>[2x]QLTIEVLVTVDGVNFRTVVLNNKNTYRSQLGCVFFNGADISDTIPDEKQNGHSLYLADNLTADETKALKELYGPVDPTFLHRFYSLKAAVHGWKMVVCDKVRSLKLSDNNCYLNAVIMTLDLLKDIKFVIPALQHAFMKHKGGDSTDFIALIMAYGNCTFGAPDDASRLLHTVLAKAELCCSARMVWREWCNVCGIKDVVLQGLKACCYVGVQTVEDLRA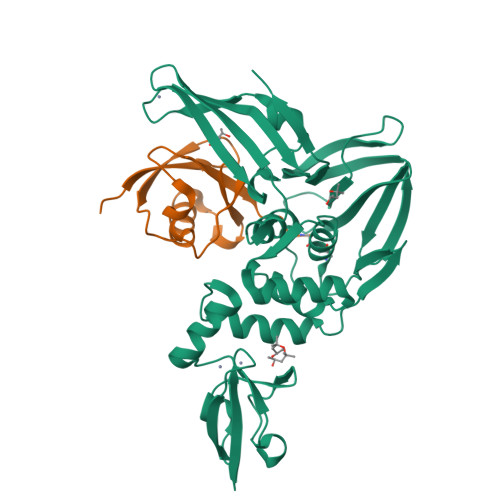RMTYVCQCGGERHRQLVEHTTPWLLLSGTPNEKLVTTSTAPDFVAFNVFQGIETAVGHYVHARLKGGLILKFDSGTVSKTSDWKCKVTDVLFPGQKYSSDCN;>MEPLSILVRNNKGRSSTYEVRLTQTVAHLKQQVSGLEGVQDDLFWLTFEGKPLEDQLPLGEYGLKPLSTVFMNLRLRG[2x]>LSSSPSEILQELGKGSTHPQPGVSPPAAPAAPGPKDGPGETDAFGNSEGKELVASGENKIKQGLLPSLEDLLFYTIAEGQEKIPVHKFITALKSTGLRTSDPRLKECMDMLRLTLQTTSDGVMLDKDLFKKCVQSNIVLLTQAF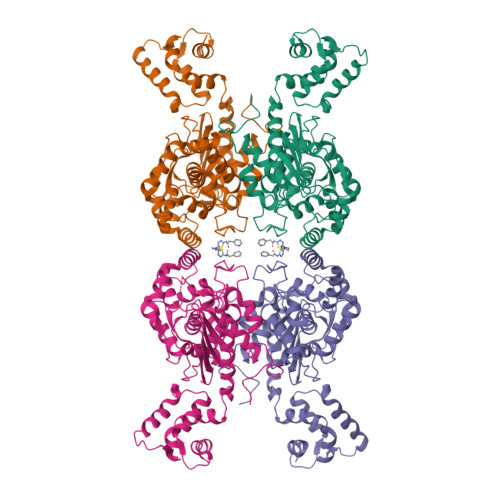RRKFVIPDFMSFTSHIDELYESAKKQSGGKVADYIPQLAKFSPDLWGVSVCTVDGQRHSTGDTKVPFCLQSCVKPLKYAIAVNDLGTEYVHRYVGKEPSGLRFNKLFLNEDDKPHNPMVNAGAIVVTSLIKQGVNNAEKFDYVMQFLNKMAGNEYVGFSNATFQSERESGDRNFAIGYYLKEKKCFPEGTDMVGILDFYFQLCSIEVTCESASVMAATLANGGFCPITGERVLSPEAVRNTLSLMHSCGMYDFSGQFAFHVGLPAKSGVAGGILLVVPNVMGMMCWSPPLDKMGNSVKGIHFCHDLVSLCNFHNYDNLRHFAKKLDPRREGGDQRHSFGPLDYESLQQELALKETVWKKVSPESNEDISTTVVYRMESLGEKS[4x]>GSMTDSEKSATIKVTDASFATDVLSSNKPVLVDFWATWCGPSKMVAPVLEEIATERATDLTVAKLDVDTNPETARNFQVVS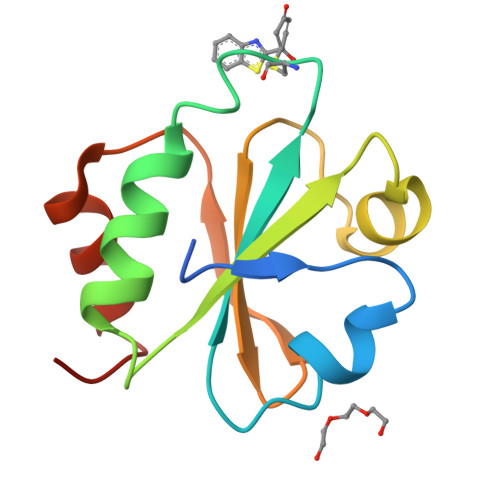IPTLILFKDGQPVKRIVGAKGKAALLRELSDVVPNLN[4x]> HHHHHHSSGENLYFQGHMAPIQDPVAFIKQMPYHQVV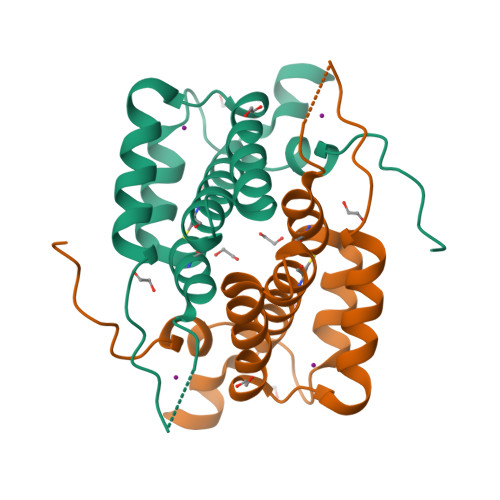KELALSRCLAQVSDSDKAFSLDAARTANAMREWMPFDIESGDEKINVLIDKYKSRINEFHSETKDKSQGVTLNCLRLYHSPELDKLSRQLIAGNPDRTWNQDNAK> PELPEVETIRRTLLPLIVGKTIEDVRIFWPNIIRHPRDSEAFAARMIGQTVRGLERRGKFLKFLLDRDALISHLRMEGRYAVASALEPLEPHTHVVFCFTDGSELRYRDVAKFGTMHVYAKE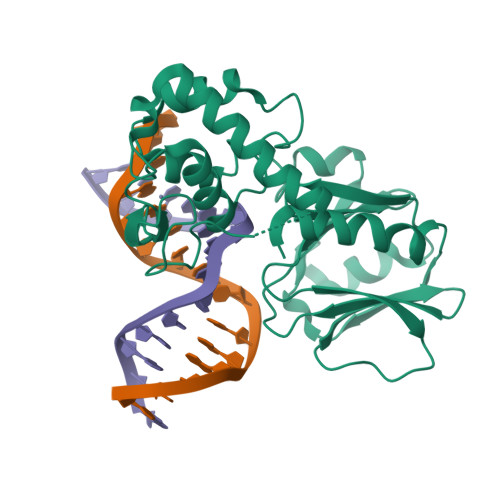EADRRPPLAELGPEPLSPAFSPAVLAERAVKTKRSVKALLLDCTVVAGFGNIYVDESLFRAGILPGRPAASLSSKEIERLHEEMVATIGEAVMKGGSTVRTYVNTQGEAGTFQHHLYVYGRQGNPCKRCGTPIEKTVVAGRGTHYCPRCQR(2R)-octane-1,2-diol | C8 H18 O2 | 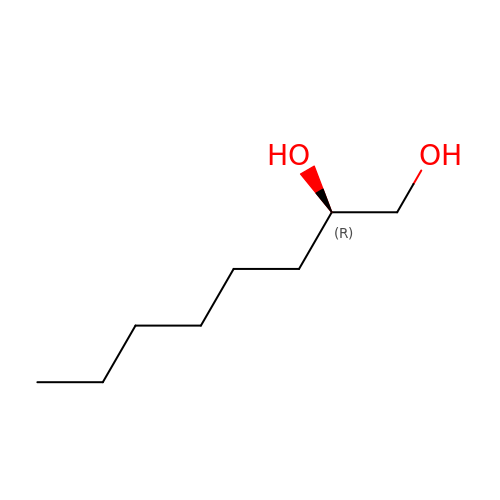AEIJTFQOBWATKX-MRVPVSSYSA-N> GELVRTDSPNFLCSVLPTHWRCNKTLPIAFKVVALGDVPDGTLVTVMAGNDENYSAELRN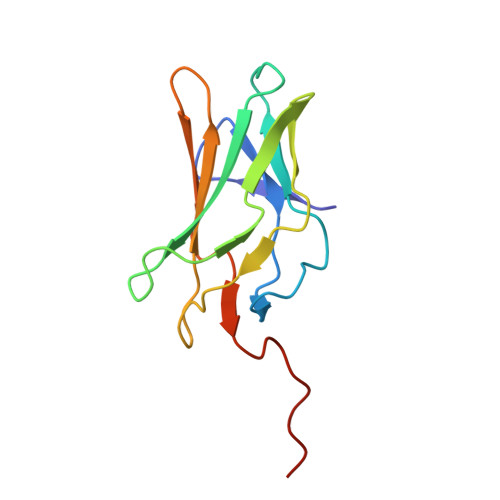ATAAMKNQVARFNDLRFVGRSGRGKSFTLTITVFTNPPQVATYHRAIKITVDGPREPRRHRQK>SNAMIVGLGTDIAEIERVEKALARSGENFARRILTDSELEQFHASKQQGRFLAKRFAAK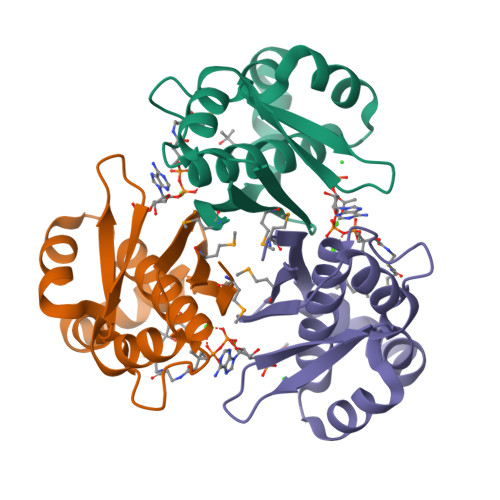EAASKALGTGIAQGVTFHDFTISHDKLGKPLLILSGQAAELASQLQVENIHLSISDERHYAMATVILERR[24x]> KIFKPEELRQALMPTLEALYRQDPESLPFRQPVDPQLLGIPDYFDIVKSPMDLSTIKRKLDTGQYQEPWQYVDDIWLMFNNAWLYNRKTSRVYKYCSKLSEVFEQEIDPVMQSLGYCCGRKLGELFVECTECGRKMHQICVLHHEIIWPAGFV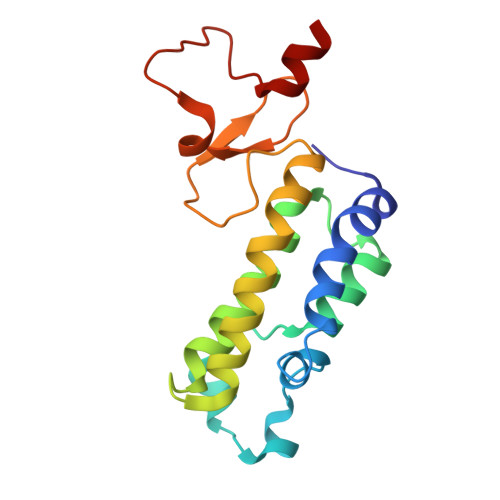CDGCLKKS>MTLHSWLDRYEKILASRGIKQKTLINYMSKIKAIRRGLPDAPLEDITTKEIAAMLNGYIDEGKAASAKLIRSTLSDAFREAIAEGHITTNHVAATRAAKSEVRRSRLTADEYLKIYQAAESSPCWLRLAMELAVVTGQRVGDLCEMKWSDIVDGYLYVEQSKTGVKIAIPTALHIDALGISMKETLDKCKEILGGETIIASTRREPLSSGTVSRYFM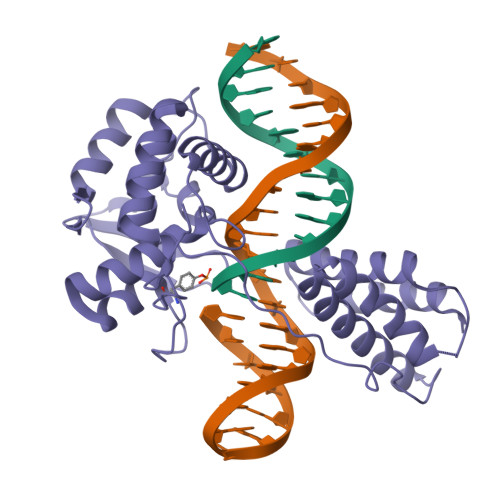RARKASGLSFEGDPPTFHELRSLSARLYEKQISDKFAQHLLGHKSDTMASQYRDDRGREWDKIEIK[2x]> MGSDKIHH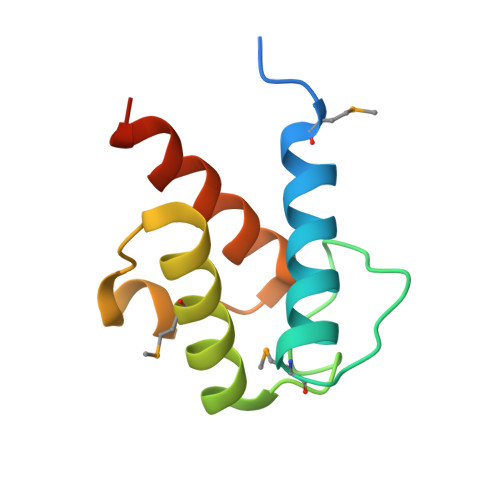HHHHMERKKLIAKFVEIASEKMGKDLETVDEENTFKELGFDSIDVIDLVMFFEDEFALRIEDEEISKIRKVKDLIDIVIKKLEEIDDEVSEG>[8x]EWQENKSWNAHFTEHKSQGVVVLWNENKQQGFTNNLKRANQ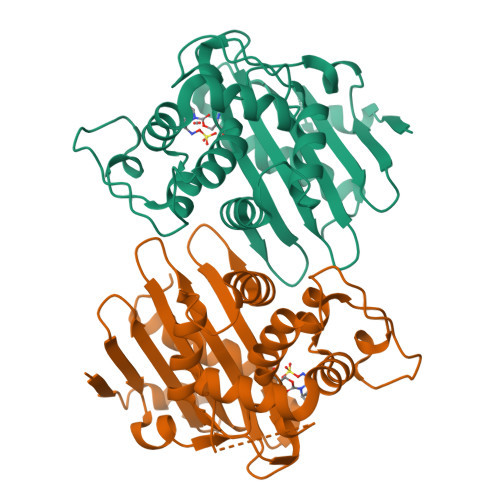AFLPASTFKIPNSLIALDLGVVKDEHQVFKWDGQTRDIATWNRDHNLITAMKYSVVPVYQEFARQIGEARMSKMLHAFDYGNEDISGNVDSFWLDGGIRISATEQISFLRKLYHNKLHVSERSQRIVKQAMLTEANGDYIIRAKTGYSTRIEPKIGWWVGWVELDDNVWFFAMNMDMPTSDGLGLRQAITKEVLKQEKIIP> GPISPIETVPVKLKPGMDGPKVKQWPLTEEKIKALVEICTEMEKEGKISKIGPENPYNTPVFA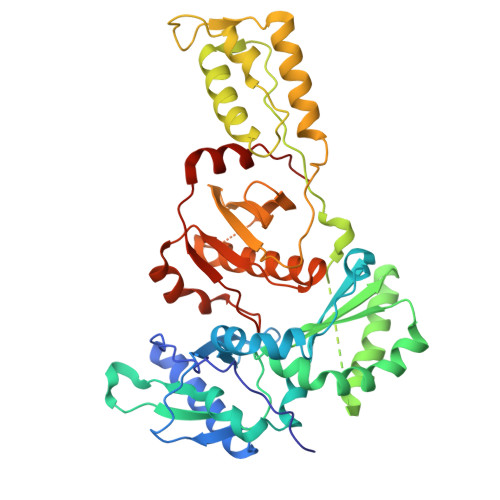IKKKDGTKWRKLVDFRELNKKTQDFWEVQLGIPHPAGLKKKKSVTVLDVGDAYFSVPLDEDFRKYTAFTIPSINNETPGIRYQYNVLPQGWKGSPAIFQSSMTKILEPFRKQNPDIVIYQYMDDLYVGSDLEIGQHRTKIEELRQHLLRWGLTTPDKKHQKEPPFLWMGYELHPDKWTVQPIVLPEKDSWTVNDIQKLVGKLNWASQIYPGIKVRQLCKLLRGTKALTEVIPLTEEAELELAENREILKEPVHGVYYDPSKDLIAEIQKQGQGQWTYQIYQEPFKNLKTGKYARMRGAHTNDVKQLTEAVQKITTESIVIWGKTPKFKLPIQKETWETWWTEYWQATWVPEWEFVNTPPLVKLWYQLEKEPIVGAETF Human Epidermal growth factor Receptor 4 (HER4 or ERBB4) carries out essential functions in the development and maintenance of the cardiovascular and nervous systems. HER4 activation is regulated by a diverse group of extracellular ligands including the neuregulin (NRG) family and betacellulin (BTC), which promote HER4 homodimerization or heterodimerization with other HER receptors. Important cardiovascular functions of HER4 are exerted via heterodimerization with its close homolog and orphan receptor, HER2. Here, we report cryo-EM structures of near full-length HER2/HER4 heterodimers and full-length HER4 homodimers bound to NRG1β and BTC.

We used this set of interface mutations to enrich for the fraction of functional HER2-G778D-V956R/HER4-I712Q heterodimers in large-scale purification for structural studies. Focused data processing on the ectodomains resulted in reconstructions of the NRG1β- and BTC-bound HER2/HER4 heterodimers at 3.3 Å and 4.3 Å resolution, respectively. In both structures, the ectodomains adopt a characteristic ‘heart-shaped’ arrangement observed in previously solved X-ray and cryo-EM structures of liganded HER receptor dimers. The conformation adopted by HER4 in our structure is identical to a previously observed conformation in the crystal structure of isolated HER4 extracellular domain bound to NRG1β (RMSD 1.7 Å – 4.4 Å across different structures). The HER2 dimerization arm is stabilized by several polar and Van-der-Waals interactions with the dimerization arm-binding pocket of HER4, which involve two conserved aromatic residues, specifically Y274 and F279 in HER2 that interact with HER4 G286, C304, and R306. The equivalent residues in the HER4 dimerization arm, Y268 and F273, are engaged in reciprocal interactions with the backbone atoms of HER2 G292, C311, and L313 via a network of hydrogen bonds. The D277 in the HER2 tip hydrogen bonds with T108 in domain I of HER4, while the T271 in the HER4 tip hydrogen bonds with T105 in HER2 domain I. The HER2/HER4 complex is the only HER2 heterodimer that involves domain I of both receptors in the dimer interface via the tip of the dimerization arms in a near-symmetric fashion. The HER2/HER4 interface has two salt bridges (HER2 H237 – HER4 D218 and HER2 E265 – HER4 R232) compared to only one in HER2/EGFR and none in HER2/HER3. However, in contrast to the HER4 homodimers, we do not observe continuous density connecting the two heterodimer monomers indicating that glycan-mediated interfaces seen in HER4 homodimers cannot be established in HER2/HER4 heterodimers.

> QSVCAGTENKLSSLSDLEQQYRALRKYYENCEVVMGNLEITSIEHNRDLSFLRSVREVTGYVLVALNQFRYLPLENLRIIRGTKLYEDRYALAIFLNYRKDGNFGLQELGLKNLTEILNGGVYVDQNKFLCYADTIHWQDIVRNPWPSNLTLVSTNGSSGCGRCHKSCTGRCWGPTENHCQTLTRTVCAEQCDGRCYGPYVSDCCHRECAGGCSGPKDTDCFACMNFNDSGACVTQCPQTFVYNPTTFQLEHNFNAKYTYGAFCVKKCPHNFVVDSSSCVRACPSSKMEVEENGIKMCKPCTDICPKACDGIGTGSLMSAQTVDSSNIDKFINCTKINGNLIFLVTGIHGDPYNAIEAIDPEKLNVFRTVREITGFLNIQSWPPNMTDFSVFSNLVTIGGRVLYSGLSLLILKQQGITSLQFQSLKEISAGNIYITDNSNLCYYHTINWTTLFSTINQRIVIRDNRKAENCTAEGMVCNHLCSSDGCWGPGPDQCLSCRRFSRGRICIESCNLYDGEFREFENGSICVECDPQCEKMEDGLLTCHGPGPDNCTKCSHFKDGPNCVEKCPDGLQGANSFIFKYADPDRECHPCHPNCTQGCNGPTSHDCI;> QVCTGTDMKLRLPASPETHLDMLRHLYQGCQVVQGNLELTYLPTNASLSFLQDIQEVQGYVLIAHNQVRQVPLQRLRIVRGTQLFEDNYALAVLDNGDPLNNTTPVTGASPGGLRELQLRSLTEILKGGVLIQRNPQLCYQDTILWKDIFHKNNQLALTLIDTNRSRACHPCSPMCKGSRCWGESSEDCQSLTRTVCAGGCARCKGPLPTDCCHEQCAAGCTGPKHSDCLACLHFNHSGICELHCPALVTYNTDTFESMPNPEGRYTFGASCVTACPYNYLSTDVGSCTLVCPLHNQEVTAEDGTQRCEKCSKPCARVCYGLGMEHLREVRAVTSANIQEFAGCKKIFGSLAFLPESFDGDPASNTAPLQPEQLQVFETLEEITGYLYISAWPDSLPDLSVFQNLQVIRGRILHNGAYSLTLQGLGISWLGLRSLRELGSGLALIHHNTHLCFVHTVPWDQLFRNPHQALLHTANRPEDECVGEGLACHQLCARGHCWGPGPTQCVNCSQFLRGQECVEECRVLQGLPREYVNARHCLPCHPECQPQNGSVTCFGPEADQCVACAHYKDPPFCVARCPSGVKPDLSYMPIWKFPDEEGACQPCPIN;> SHLVKCAEKEKTFCVNGGECFMVKDLSNPSRYLCKCPNEFTGDRCQNYVMAS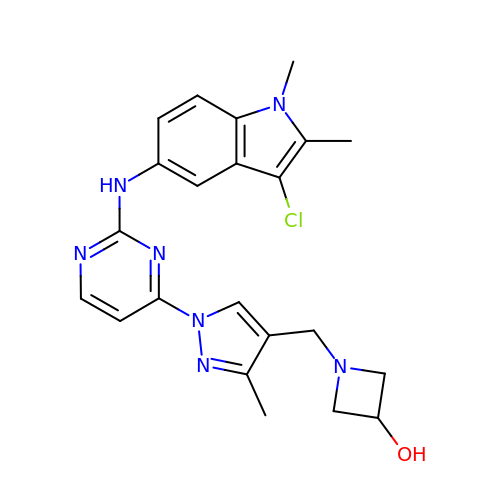1-[(1-{2-[(3-chloro-1,2-dimethyl-1H-indol-5-yl)amino]pyrimidin-4-yl}-3-methyl-1H-pyrazol-4-yl)methyl]azetidin-3-ol | C22 H24 Cl N7 O | XHZDAKAAKUZJHY-UHFFFAOYSA-N> GPAMNSVFSGLDMLILLPYERRGTRLVVEDYRPDHIYCIGADFGKNQDYSVFSVLDLDTGAIACLERMNGATWSDQVARLKALSEDYGHAYVVADTWGVGDAIAEELDAQGINYTPLPVKSSSVKEQLISNLALLMEKGQVAVPNDKTILDELRNFRYYRTASGNQVMRAYGRGHDDIVMSLALAYSQYEG

The large terminase protein is a key component of the DNA packaging machinery in tailed bacteriophages and evolutionarily related herpes viruses. Typically, in addition to an ATPase domain which powers DNA translocation, the large terminase contains a nuclease domain which cuts concatemeric DNA, generated by rolling circle replication. Crystal structures of the large terminase nuclease from the thermophilic bacteriophage G20c show that it is most similar to the RuvC family of the RNase H-like endonucleases. The overall structure adopts the RNase-H fold.

Subsequently a recombinant protein construct, residues 257 to 443, corresponding to the nuclease domain, crystallized in two different crystal forms, 2 and 3. Crystal forms 1 and 2 contain a single molecule, whereas crystal form 3 contains two protein molecules per asymmetric unit. The two other loops, L0 and L3, residues 295–301 and 423–427, respectively, also contribute to the active site. The β-hairpin (β9 and β10 strands on Figure 1A), a unique feature of viral large terminases not observed in other members of the RNase H-like endonucleases, is well ordered in crystal forms 2 and 3, but is invisible in the structure of the proteolytic fragment (crystal form 1). Superposition of crystal forms 1, 2 and 3 shows that four loops (L0, L1, L2, L3) surrounding the catalytic site and the β-hairpin are flexible and adopt different conformations. Importantly, all of these flexible structural segments are conserved both in phage and herpesvirus terminases. We note that D347, implicated in facilitating metal binding at site B during the catalysis (see below), is located at the N-terminus of L1. The position of this residue differs significantly between crystal forms 2 and 3, bringing the carboxyl group of D347 1.4 Å closer to the catalytic D294, which is expected to coordinate to both site A and B metals. Therefore, we suggest that D347 would coordinate metal B in a bidentate conformation, to allow formation of a similarly dehydrated and irregular coordination at metal B. Binding of metal B can be facilitated by flexibility in the position of D347, observed in the crystal structures presented here, allowing D347 to move closer to D294.>MNAQTSTATQKHRVAPPPHVPGHLIREIDAYDLDGLEQGFHEAWKRVQQPDTPPLVWTPFTGGHWIATRGTLIDEIYRSPERFSSRVIWVPREAGEAYDMVPTKLDPPEHTPYRKAIDKGLNLAEIRKLEDQIRTIAVEIIEGFADRGHCEFGSEFSTVFPVRVFLALAGLPVEDATKLGLLANEMTRPSGNTPEEQGRSLEAANKGFFEYVAPIIAARRGGSGTDLITRILNVEIDGKPMPDDRALGLVSLLLLGGLDTVVNFLGFMMIYLSRHPETVAEMRREPLKLQRGVEELFRRFAVVSDARYVVSDMEFHGTMLKEGDLILLPTALHGLDDRHHDDPMTVDLSRRDVTHSTFAQGPHRCAGMHLARLEVTVMLQEWLA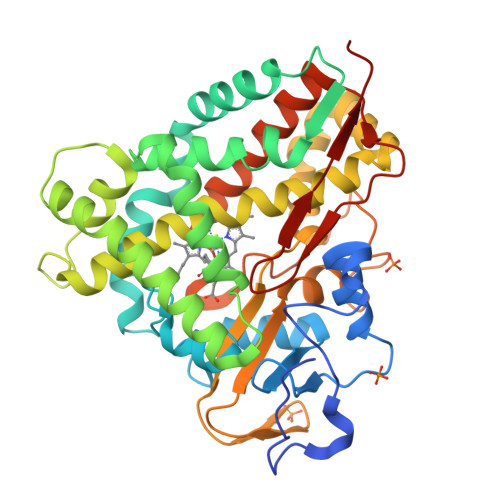RIPEFRLKDRAVPIYHSGIVAAVENIPLEWEPQRVSA[2x]> SKMSDVKCTSVVL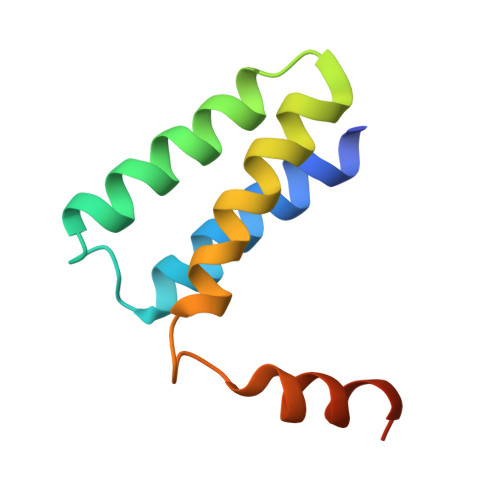LSVLQQLRVESSSKLWAQCVQLHNDILLAKDTTEAFEKMVSLLSVLLSMQGAVDINKLCEEMLDNRATLQ>FVAELNNLLGREVQVVLSNGEVYKGVLHAVDNQLNIVLANASNKAGE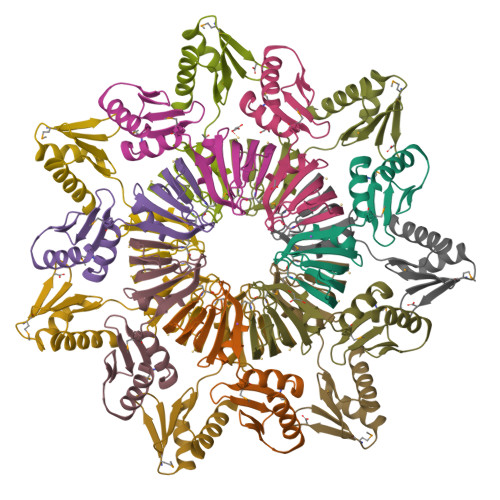KFNRVFIMYRYIVHIDSTERRIDMREFAKQAEKIFPGMVKYIEETNVVLIGDKVRVSEIGVEGVGPVAERAKRLFEEFLKRYS[28x]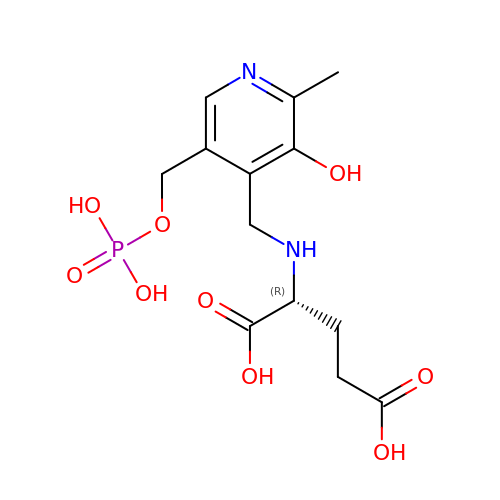N-({3-HYDROXY-2-METHYL-5-[(PHOSPHONOOXY)METHYL]PYRIDIN-4-YL}METHYL)-D-GLUTAMIC ACID | C13 H19 N2 O9 P | JMRKOGDJNHPMHS-SNVBAGLBSA-N>[2x]HHHHHQMAEEFVQQRLANNKVTI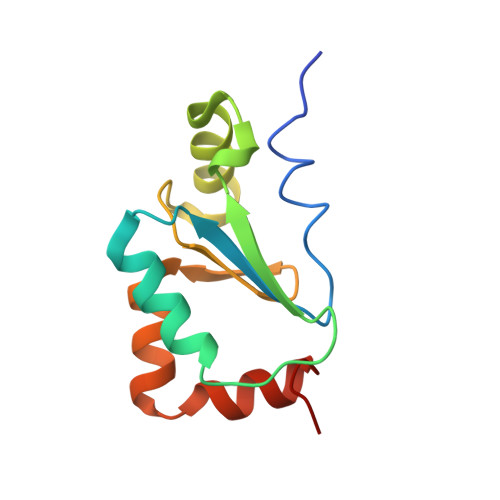FVKYTCPFCRNALDILNKFSFKRGAYEIVDIKEFKPENELRDYFEQITGGKTVPRIFFGKTSIGGYSDLLEIDNMDALGDILSSIGVLRTC NADPH oxidase 5 (NOX5) catalyzes the production of superoxide free radicals and regulates physiological processes from sperm motility to cardiac rhythm. NOX5 catalyzes the electron transfer from cytosolic NADPH to extracellular oxygen to produce superoxide (O2-) in the presence of intracellular Ca2+ ions. Like DUOX1-2, Ca2+ activates NOX5 by binding to its regulatory EF-hand domain (EFD). Each protomer contains a catalytic core with TMD, FBD and NBD and a regulatory EFD.

In the consensus structure of intermediate state (Ca2+- and NADPH-bound NOX5) determined at an overall resolution of 3.3 Å with C2 symmetry, the EFD was not resolved due to its flexibility. To analyze the EFD motion, we performed 3D classification and refinement without applying symmetry and identified at least three distinct conformations (intermediate state 1–3) with large spatial displacement. The local resolutions of EFD in intermediate state 1 and 2 are insufficient for modeling secondary structure, whereas the intermediate state 3 was resolved to an overall resolution of 3.9 Å, enabling the model building of EFD. These conformations, with the EFDs manifesting a trajectory towards the membrane, could represent its motions during NOX5 activation process. The EFD moves toward the membrane upon Ca2+ activation, shortening the distance by more than 12 Å between EFD and TMD. The preTM1 helix, which caps the NADPH-binding pocket, uplifts. The NBD shows a minor displacement coupled to the movement of the REFBD motif. These conformational changes synergistically remodel the NADPH-binding pocket by enlarging the binding site and altering the local surface potential. Finally, the nicotinamide moiety of NADPH shows a weak density in the intermediate state 3 structure, suggesting the flexibility of this moiety as observed in the mouse DUOX1 structure. In addition, the PhosR region becomes flexible and not visible upon Ca2+ binding.

>[2x]MSAEEDARWLRWVTQQFKTIAGEDGEISLQEFKAALHVKESFFAERFFALFDSDRSGTITLQELQEALTLLIHGSPMDKLKFLFQVYDIDGSGSIDPDELRTVLQSCLRESAISLPDEKLDQLTLALFESADADGNGAITFEELRDELQRFPGVMENLTISAAHWLTAPAPRPRPRRPRQLTRAYWHNHRSQLFCLATYAGLHVLLFGLAASAHRDLGASVMVAKGCGQCLNFDCSFIAVLMLRRCLTWLRATWLAQVLPLDQNIQFHQLMGYVVVGLSLVHTVAHTVNFVLQAQAEASPFQFWELLLTTRPGIGWVHGSASPTGVALLLLLLLMFICSSSCIRRSGHFEVFYWTHLSYLLVWLLLIFHGPNFWKWLLVPGILFFLEKAIGLAVSRMAAVCIMEVNLLPSKVTHLLIKRPPFFHYRPGDYLYLNIPTIARYEWHPFTISSAPEQKDTIWLHIRSQGQWTNRLYESFKASDPLGRGSKRLSRSVTMRKSQRSSKGSEILLEKHKFCNIKCYIDGPYGTPTRRIFASEHAVLIGAGIGITPFASILQSIMYRHQKRKHTCPSCQHSWIEGVQDNMKLHKVDFIWINRDQRSFEWFVSLLTKLEMDQAEEAQYGRFLELHMYMTSALGKNDMKAIGLQMALDLLANKEKKDSITGLQTRTQPGRPDWSKVFQKVAAEKKGKVQVFFCGSPALAKVLKGHCEKFGFRFFQENF> HMHHHHHHQEEDLPRPSISAEPGTVIPLGSHVTFVCRGPVGVQTFRLERESRSTY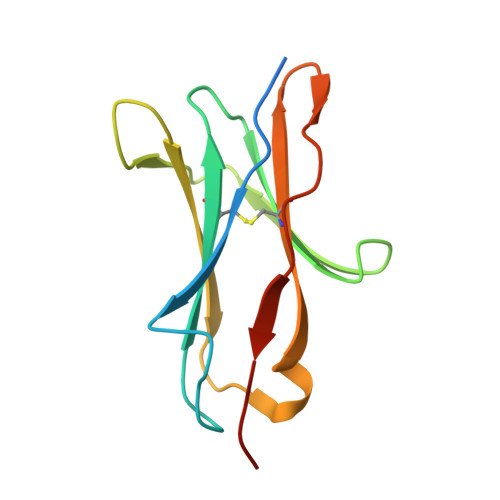NDTEDVSQASPSESEARFRIDSVSEGNAGPYRCIYYKPPKWSEQSDYLELLVKEAAA>SMQDTDNQAKIIPKPTPTPLSLESGMKGENWRKIEPENIVVITTKYGDILIELNPEFAPGHVARFQDMVKARAYNGKEFYRVIDGFVAQGGIDAEDKKWPPLEIEHEQPLLEADQIQLLDNDDLFAEKVGFLNGFPVGFDAEKKWLLHCPGMLAMARDSDPNTGGTDFYITLDAQRYLDRNMTVFGRVISGMQYVQKLQRGDKNIEGGVIQSPNKGDEMISVKLASELPENQQPNYEVMRTETAGFMNSINSKRVRSDPFFFNTPPQVVDVCDVEVPTELVDF[6x]

Hirschia baltica contains two cytosolic and five periplasmic canonical single-domain PPIases, but also two large, homologous cyclophilins with 293 and 300 residues, which we term AquaCyp293 and AquaCyp300, respectively. Our data reveal a unique two-domain architecture of AquaCyp proteins, in which the catalytically active cyclophilin domain maintains extensive contacts with a composite domain formed by terminal extensions and internal insertion elements. The crystal structures of AquaCyp293 and AquaCyp300 demonstrate that AquaCyps fold into two domains, a classical cyclophilin-type PPIase domain and the NIC domain with a novel mixed alpha-helical/beta-strand structure. Both AquaCyp proteins are stabilized by a conserved inter-domain disulfide bond.

However, AquaCyp300 elutes in SEC-MALS as a mixture of monomers (60%) and dimers (40%) when injected at a protein concentration of 1 mg/ml. AquaCyp300 is active as a PPIase as well, but it differs significantly from AquaCyp293 and human Cyp18. A moderate PPIase activity was observed only for the Leu-Pro containing peptide, pointing to pronounced substrate specificity for hydrophobic residues preceding proline. In contrast to AquaCyp293, AquaCyp300 differs from hCyp18 and EcCypB at six out of nine active site positions. The residues His54, Gln111, His126, which contribute to the PPIase activity of hCyp18 as well, are substituted by Tyr, Asp, Met, respectively, providing a plausible explanation for the low PPIase activity and high substrate specificity of AquaCyp300. In AquaCyp300, the first eight residues are not resolved in the crystal structure, presumably because they are mobile. In the AquaCyp300 crystal structure the six monomers are indeed arranged into three dimers. 50 residues form the AquaCyp300 dimer with an interface area of 1713.4 Å2 (12.9% of the molecule surface), placing the active sites of AquaCyp300 on opposing faces of the dimer. In particular, an extended hairpin structure enriched in hydrophobic residues (including three phenylalanines Phe258-Phe260) at the C-terminal extension interlocks the two monomers. To our knowledge AquaCyp300 is the first reported dimeric cyclophilin.> GKLNIVTTFYPVYEFTKQV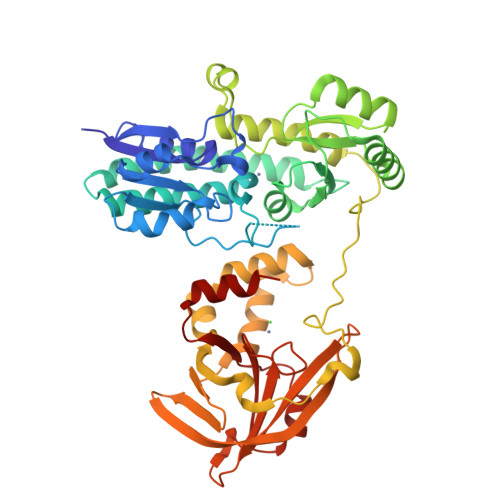AGDTANVELLIGAGTEPHEYEPSAKAVAKIQDADTFVYENENMETWVPKLLDTLDKKKVKTIKATGDMLLLPGGEEEEGDHDHGEEGHHHEFDPHVWLSPVRAIKLVEHIRDSLSADYPDKKETFEKNAAAYIEKLQSLDKAYAEGLSQAKQKSFVTQHAAFNYLALDYGLKQVAISGLSPDAEPSAARLAELTEYVKKNKIAYIYFEENASQALANTLSKEAGVKTDVLNPLESLTEEDTKAGENYISVMEKNLKALKQTTDQEGPAIEPEKAEDTKTVQNGYFEDAAVKDRTLSDYAGNWQSVYPFLEDGTFDQVFDYKAKLTGKMTQAEYKAYYTKGYQTDVTKINITDNTMEFVQGGQSKKYTYKYVGKKILTYKKGNRGVRFLFEATDADAGQFKYVQFSDHNIAPVKAEHFHIFFGGTSQETLFEEMDNWPTYYPDNLSGQEIAQEMLAH> MSNITIYHNPASGTS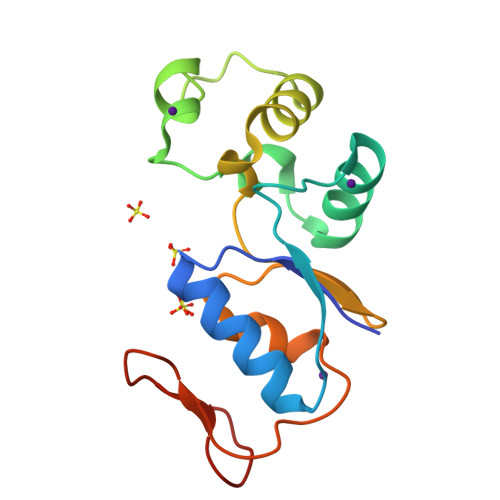RNTLEMIRNSGTEPTIILYLENPPSRDELVKLIADMGISVRALLRKNVEPYEQLGLAEDKFTDDQLIDFMLQHPILINRPIVVTPLGTRLCRPSEVVLDILQDAQKGAFTKEDGEKVVDEAGKRLK> GSH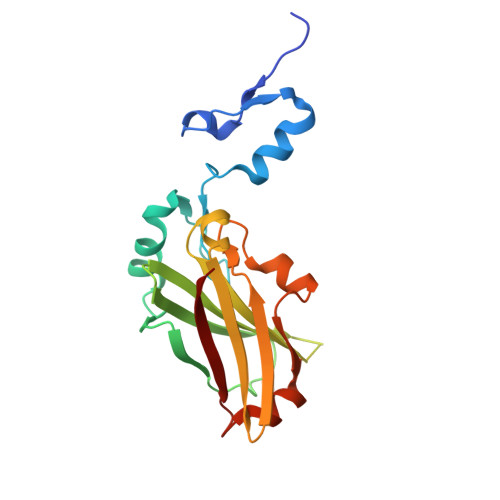VANSVLFPCKYASSGCEITLPHTEKADHEELCEFRPYSCPCPGASCKWQGSLDAVMPHLMHQHKSICTLQGEDIVFLATDINLPGAVDWVMMQSCFGFHFMLVLEKQEKYDGHQQFFAIVQLIGTRKQAENFAYRLELNGHRRRLTWEATPRSIHEGIATAIMNSDCLVFDTSIAQLFAENGNLGINVTISMC>MAHHHHHHVDDDDKMTTSPVHEQLQVPQCLAAKITVPHKILAENKEFKIIDVLSSDVETLTILADKVSCGHFVNVSHKLTGTLAANQQQSAQKLLQKKLVKPFGVSKLHKDVYEIKHEEEVNAALKEIVSDNIWQTLTHMTSYYNRSATKDTGVETANWLKSKFE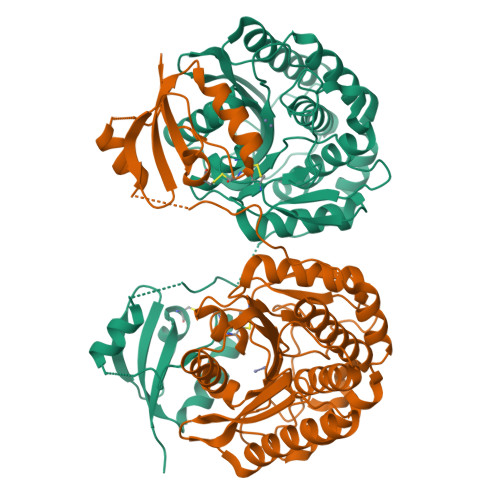QMAVEYGRTDTSTFFVKTGWYKQPSLVTVIGKDIKAPAIVIGAHMDTLDGRMPGAGDDGSGSSSIMEAARVILSSKTTFKRPIYFIWYAAEERGLVGSQHVVQHFQEQSIPVKAVVQFDMTGYRNDANDPTMWVFTDYTDRDLSNYLAKLIDHYIHVPVDYSRCGYGCSDHASWNEEDIPAAFPCETSFADHNPYIHTSSDKMDLLNLEHMTNFSKLAVAFAIELASE[2x]>[5x]ALSKVKLNDTLNKDQLLSSSKYTIQRSTGDSIDTPNYDVQKHINKLCGMLLITEDANHKFTGLIGMLYAMSRLGREDTIKILRDAGYHVKANGVDVTTHRQDINGKEMKFEVLTLASLTTEIQINIEIESRKSYKKMLKEMGEVAPEYRHDSPDCGMIILCIAALVITKLAAGDRSGLTAVIRRANNVLKNEMKRYKGLLPKDIANSFYEVFEKHPHFIDVFVHFGIAQSSTRGGSRVEGIFAGLFMNAYGAGQVMLRWGVLAKSVKNIMLGHASVQAEMEQVVEVYEYAQKLGGEAGFYHILNNPKASLLSLTQFPHFSSVVLGNAAGLGIMGEYRGTPRNQDLYDAAKAYAEQLKENGVINYSVLDLTAEELEAIK

HRSV belongs to the Mononegavirales order with the non-segmented negative-strand RNA genome fully coated by the viral nucleoprotein N. The resulting helical nucleocapsid (NC) shields the viral genetic material from recognition by the innate immune system while serving as template for replication and transcription by the viral RNA polymerase complex, thereby constituting a potential drug target. The helical HRSV nucleocapsid is a template for the viral RNA synthesis and a scaffold for the virion assembly. The helical NC, together with the RNA polymerase L, its phosphoprotein cofactor P and the transcription factor M2-1, form the HRSV RNA synthesis complex that constitues the minimal infectious unit of the virus. We explore the polymorphism of the nucleocapsid-like assemblies, report five structures of the full-length particles and two alternative arrangements formed by a C-terminally truncated nucleoprotein mutant, and demonstrate the functional importance of the identified longitudinal interfaces.

Indeed, the HRSV NC reveals itself as a right-handed “super-helix”, defined by a 105.3 Å rise and a 149.5° twist, generated by helical repetition of asymmetric units composed of 16 N protomers forming a ~1.5 turns left-handed spiral staircase. Indeed, an additional 3D refinement within a mask enclosing ~1.5 turns resulted in a 3.5 Å average resolution map of a five protomer-subsection in the middle of the mask, which however rapidly deteriorates towards the mask periphery due to a progressive loss of regularity. The structure of the N-RNA protomer is again largely the same as in the crystal, with RMSD less than 1 Å over 378 backbone residues for each of the five protomers, and the inter-protomer contacts maintained. The variation of the protomer tilt is visible even on the five protomer-subsection of the helix. Another striking observation is that three consecutive “nearly standing” protomers in the lower turn interact with the upper turn through their CTD-arms, which are therefore better defined than in the other protomers where they are not constrained. Indeed, inspection of the CTD-arm densities in the five protomer-subsection and in the entire asymmetric unit shows that the definition of the CTD-arm of each protomer Ni depends on the position and orientation of the protomer(s) located immediately above (i.e., Ni+10, Ni+11 and Ni+12). Although modelling of the CTD-arm after the residue 3796 would be unreliable, a rigid body fit into the subsection map indicates that the three “nearly standing” subunits of the helical HRSV NCs do show densities extending beyond.> MASMTGGQQMGRGSSGSPGVEQHTQAFLEALEQGGGKPLEQLSPKDARAVLTGAQASVKVDLSGIEVKERTIQANGQSIKLQVVRPANVKGELPVFMFFHGGGWVLGDFPTHQRLIRDLVVGSGAVAVYVDYTPSPESHYPTAINQAYAATQWVAEHGKEIGVDGKRLAVAGNAVGGNMAAVVALKAKEAGTPALRFQLLLHPVTDASFETASYKQFADGHFLTTGMMKWFWDNYTTDAKAREQIYASPLRASSEQLKGLPPALVQTAEFD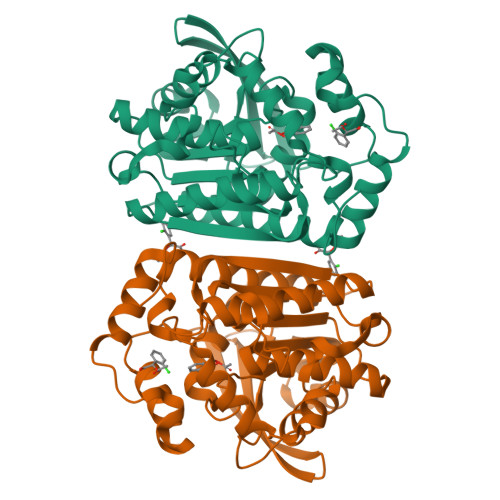VLRDEGEAYARKLNAAGVTVTSVRYNGMIHDYGLLNPLSQVPAVKAAMRQAGTELKVHLQLELEHHHHHH> XXXXXXXXXXXXXXXXXXXXXXXXXXXXXXXXXXXXXXXXXXXXXXXXXXXXXXXXXXXXXXXXXXXXXXXXXXXXXXXXXXXXXXXXXXXXXXXXXXXXXXXXXXXXXXXXXXXXXXXXXXXXXXXXXXXXXXXXXXXXXXXXXXXXXXXXXXXXXXXXXXXXXXXXXXXXXXXXXXXXXXXXXXXXXXPSVPECFTIEKKSSYFIIEPQDLSTKVASICGVIVPKVHTIHDKVFYPLTFVPTHKTVSSLRQLGRKIQNSTPIMLIGKAGSGKTFLINELSKYMGCHDSIVKIHLGEQTDAKLLIGTYTSGDKPGTFEWRAGVLATAVKEGRWVLIEDIDKAPTDVLSILLSLLEKRELTIPSRGETVKAANGFQLISTVRINEDHQKDSSNKIYNLNMIGMRIWNVIELEEPSEEDLTHILAQKFPILTNLIPKLIDSYKNVKSIYMNTKFISLNKGAHTRVVSVRDLIKLCERLDILFKNNGINKPDQLIQSSVYDSIFSEAADCFAGAIGEFKALEPIIQAIGESLDIASSRISLFLTQHVPTLENLDDSIKIGRAVLLKEKLNIQKKSMNSTLFAFTNHSLRLMEQISVCIQMTEPVLLVGETGTGKTTVVQQLAKMLAKKLTVINVSQQTETGDLLGGYKPVNSKTVAVPIQENFETLFNATFSLKKNEKFHKMLHRCFNKNQWKNVVKLWNEAYKMAQSILKITNTENENENAKKKKRRLNTHEKKLLLDKWADFNDSVKKFEAQSSSIENSFVFNFVEGSLVKTIRAGEWLLLDEVNLATADTLESISDLLTEPDSRSILLSEKGDAEPIKAHPDFRIFACMNPATDVGKRDLPMGIRSRFTEIYVHSPERDITDLLSIIDKYIGKYSVSDEWVGNDIAELYLEAKKLSDNNTIVDGSNQKPHFSIRTLTRTLLYVTDIIHIYGLRRSLYDGFCMSFLTLLDQKSEAILKPVIEKFTLGRLKNVKSIMSQTPPSPGPDYVQFKHYWMKKGPNTIQEQAHYIITPFVEKNMMNLVRATSGKRFPVLIQGPTSSGKTSMIKYLADITGHKFVRINNHEHTDLQEYLGTYVTDDTGKLSFKEGVLVEALRKGYWIVLDELNLAPTDVLEALNRLLDDNRELFIPETQEVVHPHPDFLLFATQNPPGIYGGRKILSRAFRNRFLELHFDDIPQDELEIILRERCQIAPSYAKKIVEVYRQLSIERSASRLFEQKNSFATLRDLFRWALRDAVGYEQLAASGYMLLAERCRTPQEKVTVKKTLEKVMKVKLDMDQYYASLEDKSLEAIGSVTWTKGMRRLSVLVSSCLKNKEPVLLVGETGCGKTTICQLLAQFMGRELITLNAHQNTETGDILGAQRPVRNRSEIQYKLIKSLKTALNIANDQDVDLKELLQLYSKSDNKNIAEDVQLEIQKLRDSLNVLFEWSDGPLIQAMRTGNFFLLDEISLADDSVLERLNSVLEPERSLLLAEQGSSDSLVTASENFQFFATMNPGGDYGKKELSPALRNRFTEIWVPSMEDFNDVNMIVSSRLLEDLKDLANPIVKFSEWFGKKLGGGNATSGVISLRDILAWVEFINKVFPKIQNKSTALIQGASMVFIDALGTNNTAYLAENENDLKSLRTECIIQLLKLCGDDLELQQIETNEIIVTQDELQVGMFKIPRFPDAQSSSFNLTAPTTASNLVRVVRAMQVHKPILLEGSPGVGKTSLITALANITGNKLTRINLSEQTDLVDLFGADAPGERSGEFLWHDAPFLRAMKKGEWVLLDEMNLASQSVLEGLNACLDHRGEAYIPELDISFSCHPNFLVFAAQNPQYQGGGRKGLPKSFVNRFSVVFIDMLTSDDLLLIAKHLYPSIEPDIIAKMIKLMSTLEDQVCKRKLWGNSGSPWEFNLRDTLRWLKLLNQYSICEDVDVFDFVDIIVKQRFRTISDKNKAQLLIEDIFGKFSTKENFFKLTEDYVQINNEVALRNPHYRYPITQNLFPLECNVAVYESVLKAINNNWPLVLVGPSNSGKTETIRFLASILGPRVDVFSMNSDIDSMDILGGYEQVDLTRQISYITEELTNIVREIISMNMKLSPNATAIMEGLNLLKYLLNNIVTPEKFQDFRNRFNRFFSHLEGHPLLKTMSMNIEKMTEIITKEASVKFEWFDGMLVKAVEKGHWLILDNANLCSPSVLDRLNSLLEIDGSLLINECSQEDGQPRVLKPHPNFRLFLTMDPKYGELSRAMRNRGVEIYIDELHSRSTAFDRLTLGFELGENIDFVSIDDGIKKIKLNEPDMSIPLKHYVPSYLSRPCIFAQVHDILLLSDEEPIEESLAAVIPISHLGEVGKWANNVLNCTEYSEKKIAERLYVFITFLTDMGVLEKINNLYKPANLKFQKALGLHDKQLTEETVSLTLNEYVLPTVSKYSDKIKSPESLYLLSSLRLLLNSLNALKLINEKSTHGKIDELTYIELSAAAFNGRHLKNIPRIPIFCILYNILTVMSENLKTESLFCGSNQYQYYWDLLVIVIAALETAVTKDEARLRVYKELIDSWIASVKSKSDIEITPFLNINLEFTDVLQLSRGHSITLLWDIFRKNYPTTSNSWLAFEKLINLSEKFDKVRLLQFSESYNSIKDLMDVFRLLNDDVLNNKLSEFNLLLSKLEDGINELELISNKFLNKRKHYFADEFDNLIRYTFSVDTAELIKELAPASSLATQKLTKLITNKYNYPPIFDVLWTEKNAKLTSFTSTIFSSQFLEDVVRKSNNLKSFSGNQIKQSISDAELLLSSTIKCSPNLLKSQMEYYKNMLLSWLRKVIDIHVGGDCLKLTLKELCSLIEEKTASETRVTFAEYIFPALDLAESSKSLEELGEAWITFGTGLLLLFVPDSPYDPAIHDYVLY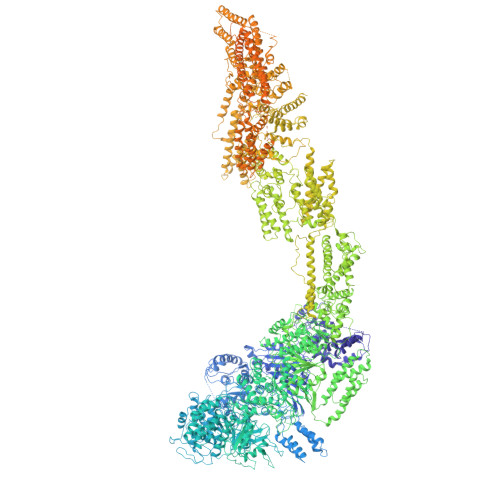DLFLKTKTFSQNLMKSWRNVRKVISGDEEIFTEKLINTISDDDAPQSPRVYRTGMSIDSLFDEWMAFLSSTMSSRQIKELVSSYKCNSDQSDRRLEMLQQNSAHFLNRLESGYSKFADLNDILAGYIYSINFGFDLLKLQKSKDRASFQISPLWSMDPINISCAENVLSAYHELSRFFKKGDMEDTSIEKVLMYFLTLFKFHKRDTNLLEIFEAALYTLYSRWSVRRFRQEQEENEKSNMFKFNDNSDDYEADFRKLFPDYEDTALVTNEKDISSPENLDDIYFKLADTYISVFDKDHDANFSSELKSGAIITTILSEDLKNTRIEELKSGSLSAVINTLDAETQSFKNTEVFGNIDFYHDFSIPEFQKAGDIIETVLKSVLKLLKQWPEHATLKELYRVSQEFLNYPIKTPLARQLQKIEQIYTYLAEWEKYASSEVSLNNTVKLITDLIVSWRKLELRTWKGLFNSEDAKTRKSIGKWWFYLYESIVISNFVSEKKETAPNATLLVSSLNLFFSKSTLGEFNARLDLVKAFYKHIQLIGLRSSKIAGLLHNTIKFYYQFKPLIDERITNGKKSLEKEIDDIILLASWKDVNVDALKQSSRKSHNNLYKIVRKYRDLLNGDAKTIIEAGLLYXXXXXXXXXXXXXXXXXXXXXXXXXXXXXXXXRNIDTVASNMDSYLEKISSQEFPNFADLASDFYAEAERLRKETPNVYTKENKKRLAYLKTQKSKLLGDALKELRRIGLKVNFREDIQKVQSSTTTILANIAPFNNEYLNSSDAFFFKILDLLPKLRSAASNPSDDIPVAAIERGMALAQSLMFSLITVRHPLSEFTNDYCKINGMMLDLEHFTCLKGDIVHSSLKANVDNVRLFEKWLPSLLDYAAQTLSVISKYSATSEQQKILLDAKSTLSSFFVHFNSSRIFDSSFIESYSRFELFINELLKKLENAKETGNAFVFDIIIEWIKANKGGPIKKEQKRGPSVEDVEQAFRRTFTSIILSFQKVIGDGIESISETDDNWLSASFKKVMVNVKLLRSSVVSKNIETALSLLKDFDFTTTESIYVKSVISFTLPVITRYYNAMTVVLERSRIYYTNTSRGMYILSTILHSLAKNGFCSPQPPSEEVDDKNLQEGTGLGDGEGAQNNNKDVEQDEDLTEDAQNENKEQQDKDERDDENEDDAVEMEGDMAGELEDLSNGEENDDEDTDSEEEELDEEIDDLNEDDPNAIDDKMWDDKASDNSKEKDTDQNLDGKNQEEDVQAAENDEQQRDNKEGGDEDPNAPEDGDEEIENDENAEEENDVGEQEDEVKDEEGEDLEANVPEIETLDLPEDMNLDSEHEESDEDVDMSDGMPDDLNKEEVGNEDEEVKQESGIESDNENDEPGPEEDAGETETALDEEEGAEEDVDMTNDEGKEDEENGPEEQAMSDEEELKQDAAMEENKEKGGEQNTEGLDGVEEKADTEDIDQEAAVQQDSGSKGAGADATDTQEQDDVGGSGTTQNTYEEDQEDVTKNNEESREEATAALKQLGDSMKEYHRRRQDIKEAQTNGEEDENLEKNNERPDEFEHVEGANTETDTQALGSATQDQLQTIDEDMAIDDDREEQEVDQKELVEDADDEKMDIDEEEMLSDIDAHDANNDVDSKKSGFIGKRKSEEDFENELSNEHFSADQEDDSEIQSLIENIEDNPPDASASLTPERSLEESRELWHKSEISTADLVSRLGEQLRLILEPTLATKLKGDYKTGKRLNMKRIIPYIASQFRKDKIWLRRTKPSKRQYQIMIALDDSKSMSESKCVKLAFDSLCLVSKTLTQLEAGGLSIVKFGENIKEVHSFDQQFSNESGARAFQWFGFQETKTDVKKLVAESTKIFERARAMVHNDQWQLEIVISDGICEDHETIQKLVRRARENKIMLVFVIIDGITSNESILDMSQVNYIPDQYGNPQLKITKYLDTFPFEFYVVVHDISELPEMLSLILRQYFTDLASS> MSLYTFKELKRATKQDTVSLPKLKVALLGDTATQLLATAIKGEGILRNYNIELWEAEYNQVERQIMDPTSDYYQFEPDYTIIFHSTHKLLEKHSLVNSDLQNKLADDRLDFVRLLCEQGIGRVIYYNYPEIEDTIWGSYATKVQSSFTYQLTKLNYELMNISQAYPNFFICNLAGISAKYGRNFMFDSSVYVNTEIILSLDALPIISSRTIDIIAAIQGKFKKCLILDLDNTIWGGVVGDDGWENIQVGHGLGIGKAFTEFQEWVKKLKNRGIIIAVCSKNNEGKAKEPFERNPEMVLKLDDIAVFV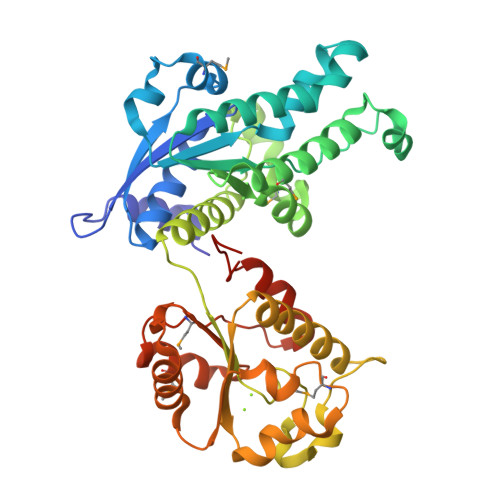ANWENKADNIRTIQRTLNIGFDSMVFLDDNPFERNMVREHVPGVTVPELPEDPGDYLEYLYTLNLFETASFSEGHHHHHH> MEQNPQSQLKLLVTRGKEQGYLTYAEVNDHLPEDIVDSDQIEDIIQMINDMGIQVMEEAPDADDLMLAENTADEDAAEAAAQVLSSVESEIGRTTDPVRMYMREMGTVELLTREGEIDIAKRIEDGINQVQCSVAEYPEAITYLLEQYDRVEAEEARLSDLITGFVDPNAEEDLAPTATHVGSELSQEDLDDDEDEDEEDGDDDSADDDNSIDPELAREKFAELRAQYVVTRDTI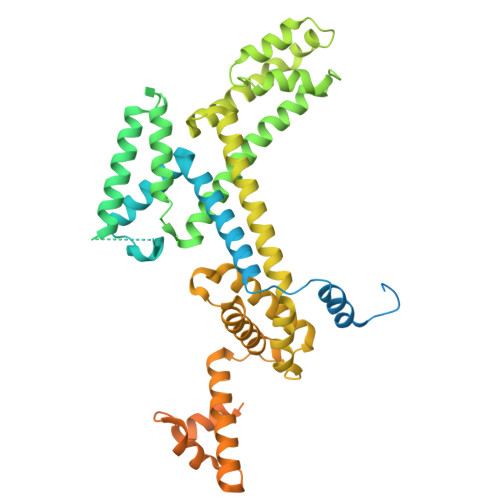KAKGRSHATAQEEILKLSEVFKQFRLVPKQFDYLVNSMRVMMDRVRTQERLIMKLCVEQCKMPKKNFITLFTGNETSDTWFNAAIAMNKPWSEKLHDVSEEVHRALQKLQQIEEETGLTIEQVKDINRRMSIGEAKARRAKKEMVEANLRLVISIAKKYTNRGLQFLDLIQEGNIGLMKAVDKFEYRRGYKFSTYATWWIRQAITRSIADQARTIRIPVHMIETINKLNRISRQMLQEMGREPTPEELAERMLMPEDKIRKVLKIAKEPISMETPIGDDEDSHLGDFIEDTTLELPLDSATTESLCAATHDVLAGLTAREAKVLRMRFGIDMNTDYTLEEVGKQFDVTRERIRQIEAKALRKLRHPSRSEVPRSFLDD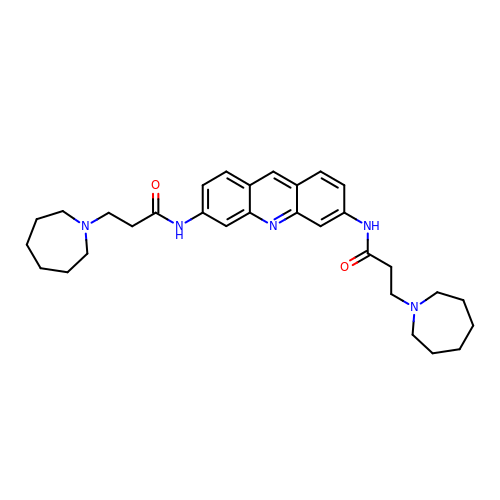3,6-Bis[3-(azepan-1-yl)propionamido]acridine | C31 H41 N5 O2 | MSWYQCALXGGGBX-UHFFFAOYSA-N>MVEDILAPGLRVVFCGINPGLSSAGTGFPFAHPANRFWKVIY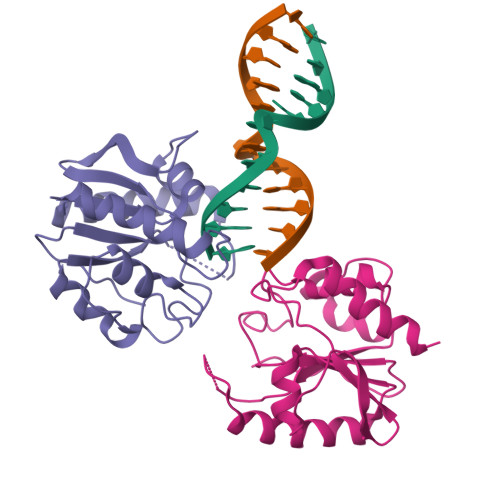QAGFTDRQLKPQEAQHLLDYRCGVTKLVDRPTVQANEVSKQELHAGGRKLIEKIEDYQPQALAILGKQAYEQGFSQRGAQWGKQTLTIGSTQIWVLPNPSGLSRVSLEKLVEAYRELDQALVVRGR[2x]>MKKLFLVFWWHMHQPLYREPYTGEYLLPWTFFHAVKDYYDMPAYLKDFEIKLNFNLTPVLIDQIQEYAQGKAKDVFLEAIRKDPDDLEKEEVEKLIEFTKLNYEKPIYRFERIRELMNKEKLNREELLDLQTLNLLAWCGRTLRKDLKDLLNKGRNYTQEEKEYVLNKYFEIIKKTLSIYREIKEEGKGSVSTSPYYHPLIPILLNPNCVYETTPNVKIPDFAVSFREDASKHVELAKEKYFEIFGEHPVYMWPPLASVSNEALELY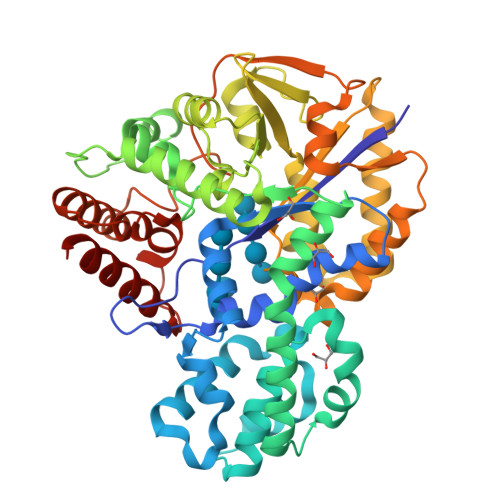YEKGINMLATDEVILKNSVERASPYLRYYFRELISVFFRDKTLSDLIGFSYHAWNAEDAVRDFIGRLKKIHESVDFQPVVFVVLDGENCWEYYEENGIPFLEKLYSTLEKEEWIETLTLEEAMRKEDVKTEVIESVKAGTWFDGNFLKWIGNKEKNEYWKILIEAKKKAKNDYILVAEGSDWFWWQGEEKAPFVEVFDKLFRSFVRRAQE[2x]> GTMAAAAVVAATVPAQSMGADGASSVHWFRKGLRLHDNPALLAAVRGARCVRCVYILDPWFAASSSVGINRWRFLLQSLEDLDTSLRKLNSRLFVVRGQPADVFPRLFKEWGVTRLTFEYDSEPFGKERDAAIMKMAKEAGVEVVTENSHTLYDLDRIIELNGQKPPLTYKRFQALISRMELPKKPAVAVSSQQMESCRAEIQENHDDTYGVPSLEELGFPTEGLGPAVWQGGETEALARLDKHLERKAWVANYERPRMNANSLLA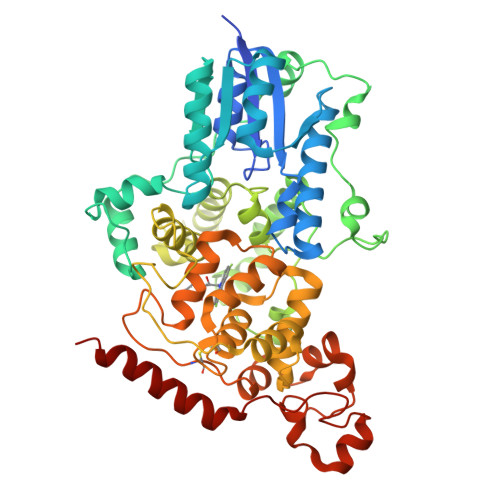SPTGLSPYLRFGCLSCRLFYYRLWDLYKKVKRNSTPPLSLFGQLLWREFFYTAATNNPRFDRMEGNPICIQIPWDRNPEALAKWAEGKTGFPWIDAIMTQLRQEGWIHHLARHAVACFLTRGDLWVSWESGVRVFDELLLDADFSVNAGSWMWLSCSAFFQQFFHCYCPVGFGRRTDPSGDYIRRYLPKLKGFPSRYIYEPWNAPESVQKAAKCIIGVDYPRPIVNHAETSRLNIERMKQIYQQLSRY DNPH1 is a 2’-deoxynucleoside 5’-phosphate N-hydrolase. It hydrolyses dNMP to form a free nucleobase moiety and 2-deoxyribose 5-phosphate. DNPH1 is a potential target for anti-cancer therapies as it is involved in cellular proliferation and is up-regulated in several types of cancer. 6-substituted AMP including some cytokinin derivatives inhibit mammalian DNPH1s, specifically rat and human DNPH1s, with affinity in the micromolar range.

The X-Ray structures of three of these derivatives in complex with a recombinant variant of rat DNPH1 reveal the mechanism of the ligand recognition and suggest several routes for further optimization. High-resolution data were obtained for three complexes while the other ligands failed to provide us with decent crystals. The new structures were all obtained in the same monoclinic space group (P1211) that differs from the orthorhombic form previously described despite the similar conditions used to grow the crystals. Having one complex - rat DNPH1-7 - in common in the two available space groups, we could conclude that the absence of electron density for the long loop (residues 47-59) was due to its intrinsic flexibility rather than packing issue. This is in agreement with published NMR data. Similarly, the adenine moiety showed a conserved orientation constrained by the two sandwiching isoleucines I18 and I65 in the three complexes. Two main families of orientation are detected whatever the chemical derivatization (isopentenyl, furfuryl and cyclopentyl). 6-substitution points toward a hydrophobic subpocket formed by the side chain of isoleucine I18 and part of the side chain of arginine R19 while in other monomers, the substitution points rather outward and interacts mainly with isoleucine I65 and rather weakly with the glutamine Q68 in the case of compound 5. None of the tested substition can fit a buried sub-pocket to maximize additional interactions. This suggests that the few favorable interactions observed in one configuration or another (inward for 7 or 1 and outward for 5) are not sufficient to dramatically alter the binding affinity. Only the cyclopentyl group (compound 7) showed a favorable entropic contribution, although the ∆S term remains negative.

>[4x]MRRSVYFCGSIRGGREDQALYARIVSRLRRYGKVLTEHVADAELEPLGEEAAGGDQFIHEQNLNWLQQADVVVAEVTQPSLGVGYELGRAVALGKPILCLFRPQSGRVLSAMIRGAADGSRFQVWDYAEGEVETMLDRYFEAYLVEHHHHHH>MHHHHHHSPLRVALYGFGNQNKEMAKMLVERKDVEIVAVISNKSNVGKDFGEVIGLAPQGILVTAGLDAAETLRTTNPQIAMLSTLSTVGDIESQLRACAENKVNVYTIAEELTFSWTSAPEKTKEMDELFKEHNVSLIGGGFLDGACCDMARTMAAMMHKIDKLDGGLQYNVDHYGQVLAIAHGVGLSEEEFYAENGPGWTSPTSYPKSYVYNMNDWFASAFGLTVIKTEEVKTPTKAPIELYSEAIGRAIPVGQCTGMIVTATTTTEEGVIIVEKQVGKCYEDGDEDMVFMNLEGNPTGGVGFTMKNPPTPAMTNTIAIS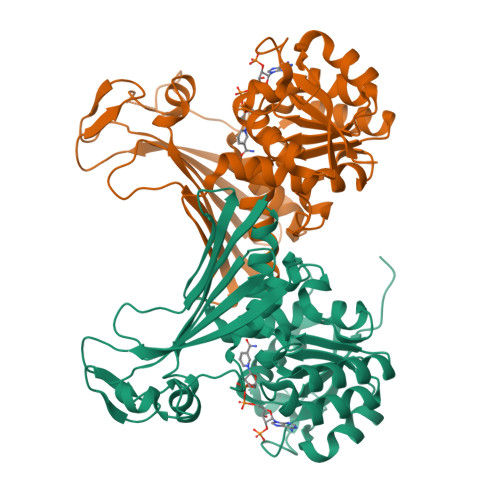RMFQTVDAPAGYITTDKLPTMEAYVHGRL[4x]>[6x]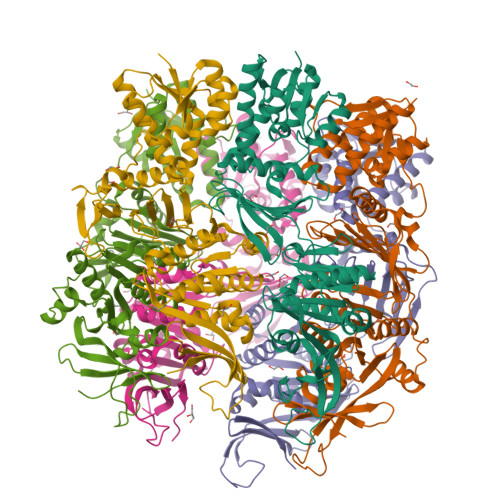MNDLMLDKSALLFGVSKYLEKGIITGNVLIHKSLLAELERESNDGLVSAEIALDEVKKLKDITERILVNFEIVGDDSKKGEANELSREYCLEKGCIIVTADETQKKICDAMGIQYNFLQPLKQGLSFESFFDDETMSLHIKEDTVPRAKKGKPGNWKFVNLSDKPMLSTDVRMIANEIINAVRLIKGSFVEIERRGSLIIQLGNYRVVITRPPLSDGWEITITRPVVRKRLEDYNLDERLIKRLEERAEGIIIAGAPGMGATTFAQALAEYYMRLGKIVKTIESPRDMHLPPEITQYSKNYAEIGELHDILLLSRPDYTVYDEMRNDEDFKLYVDLRLAGVGMVGVVHATSPIDAIHRFVNRVDIGTIPNILDTIIFINSGNVSKVYTLEMTVKVPAGLKEADLARPVVEIKDLATGNTEYEIYVFGEQTMIVPVNRGITMSNMEFKISKIVNNIIPNATVKYEDGEYVIVIPKEEIGKYNRKLVQRLKRLEKKNNIKIKIKLSD> MRNLDFIDSFIPTEGKYIRVMDFYNSEYPFCIHAPSAPNGDIMTEICSRENNQYFIFFPTDDGRVIIANRHNGSVFTGEATSVVSDIYTGSPLQFFREVKRTMATYYLAIQNP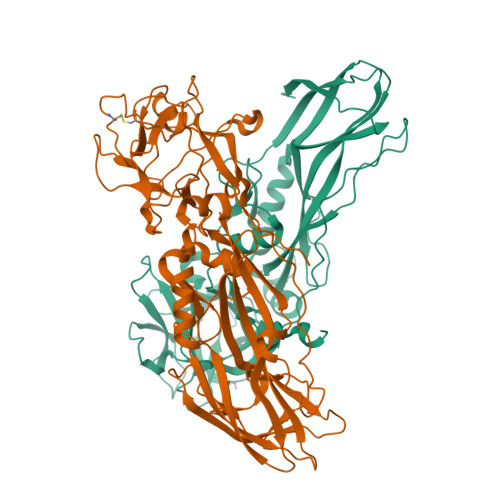ESATDVRALEPHSHELPSRLYYTNNIENNSNILISNKEQIYLTLPSLPENEQYPKTPVLSGIDDIGPNQSEKSIIGSTLIPCIMVSDFISLGERMKTTPYYYVKHTQYWQSMWSALFPPGSKETKTEKSGITDTSQISMTDGINVSIGADFGLRFGNKTFGIKGGFTYDTKTQITNTSQLLIETTYTREYTNTENFPVRYTGYVLASEFTLHRSDGTQVNTIPWVALNDNYTTIARYPHFASEPLLGNTKIITDDQN;> MCDSKDNSGVSEKCGKKFTNYPLNTTPTSLNYNLPEISKKFYNLKNKYSRNGYGLSKTEFPSSIENCPSNEYSIMYDNKDPRFLIRFLLDDGRYIIADRDDGEVFDEAPTYLDNNNHPIISRHYTGEERQKFEQVGSGDYITGEQFFQFYTQNKTRVLSNCRALDSRTILLSTAKIFPIYPPASETQLTAFVNSSFYAAAIPQLPQTSLLENIPEPTSLDDSGVLPKDAVRAVKGSALLPCIIVHDPNLNNSDKMKFNTYYLLEYKEYWHQLWSQIIPAHQTVKIQERTGISEVVQNSMIEDLNMYIGADFGMLFYFRSSGFKEQITRGLNRPLSQTTTQLGERVEEMEYYNSNDLDVRYVKYALAREFTLKRVNGEIVKNWVAVDYRLAGIQSYPNAPITNPLTLTKHTIIRCENSYDGHIFKTPLIFKNGEVIVKTNEELIPKINQ Hence, spy49_0662 was expressed with a 1.4 kDa C-terminal V5 epitope tag used for Western blotting followed by a His6-tag for immobilized metal ion affinity purification, and the resulting protein was coined as HupZ (heme utilization protein Z). The tagged HupZ is a small-sized protein previously shown to bind heme, and it exhibits a trace heme degrading activity in the presence of NADPH and cytochrome P450 reductase (CPR). This protein shares some protein sequence similarity to the members of the IsdG family. In summary, a comprehensive biochemical, spectroscopic, and structural characterization led us to propose that the observed heme binding in HupZ is through its His6-tag in a sandwiched di-heme complex from two subunits with an oxygen-derived bridging ligand.

Next, HupZ was crystallized in the primitive orthorhombic space group of P212121, and the structure was refined to 1.7-Å resolution with one dimer in an asymmetric unit. In this new structure, six and seven additional C-terminal residues are present in Chains A and B, respectively, compared to the previous structure. The C-terminal region, including the His6-tag, still misses density for 39–40 residues. Comparing the structure of H111A to the wild-type structure, the two superimpose well with an r.m.s.d value of 0.99 Å over 237 Cα carbons, indicating site-directed mutagenesis did not induce an undesired global structural perturbation. His111, as shown in Figure 7, is located on the protein surface in the homodimeric structure. The ligand-free HupZ eluted at 18.0 mL, corresponding to a molecular weight of 36 kDa when compared to the calibration curve using the known molecular standards on the same column under the same separation conditions. The molecular weight of monomeric HupZ is 18.5 kDa, and thus it eluted as a dimer. In all experiments, the higher-order oligomeric states were observed only when heme was present, indicating that heme binding to HupZ induces oligomerization, resulting in higher-order structures. Our results indicate that each subunit of HupZ binds heme in a 1:1 ratio. Collectively, the rR data coupled with the UV–vis study indicated that the heme in the binary complex is in a six-coordinate, low-spin ferric state with at least one histidine as an axial ligand.

>[2x]MITQEMKDLINNQLAMVATVDAKGQPNIGPKRSMRLWDDKTFIYNENTDGQTRINIEDNGKIEIAFVDRERLLGYRFVGTAEIQTEGAYYEAAKKWAQGRMGVPKAVGIIHVERIFNLQSGANAGKEINSESNKGELNSKLEGKPIPNPLLGLDSTRTGHHHHHH>[2x]MATDLKASSLRALKLMHLATANDDDTDEKVIALCHQAKTPVGTTDAIFIYPRFIPIARKTLKEQGTPEIRIWTSTNFPHGNDDIDIALAETRAAIAYGADGVAVVFPYRALMAGNEQVGFDLVKACKEACAAANVLLSVIIETGELKDEALIRKASEISIKAGADHIVTSTGKVAEGATPESARIMMEVIRDMGVEKTVGFIPVGGVRTAEDAQKYLAIADELFGADWADARHYAFGA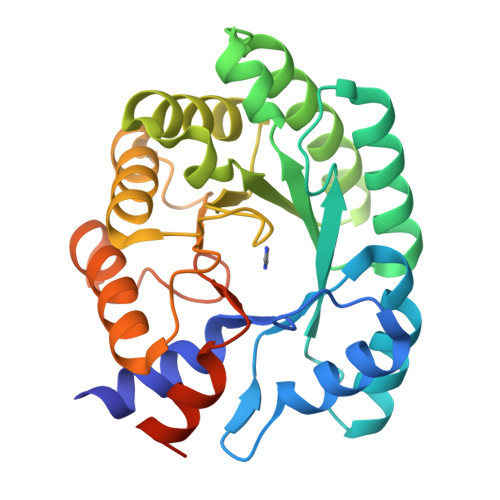SSLLASLLKALGHGDGKSASSYGSLE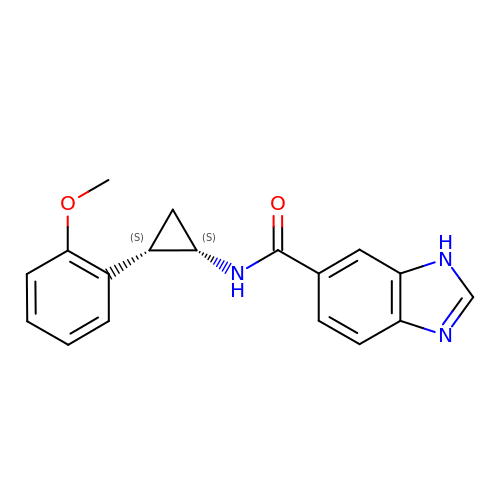~{N}-[(1~{S},2~{S})-2-(2-methoxyphenyl)cyclopropyl]-3~{H}-benzimidazole-5-carboxamide | C18 H17 N3 O2 | ZKYVGLRMGWYWNE-ZFWWWQNUSA-N>MGSSHHHHHHSSENLYFQGHSLPGANSLTIRKDSNKYVTAHFMVGIVENYTVDDWKHDMELAKETGIDAFALNCASIDSYTDKQLAYAYEAAEEVDFKVFISFDFAYWSNGDTARITSIMQTYADHPGQFQYNGAALVSTFVGDSFDWGPVKRAVDHPIFAVPNLQDPNWAGHATTSIDGAFSWYAWPTDGGNSIIKGPMTTIWDDRFRNNLKDKVYMAPVSPWFSTHFNTKNWVFICEDLPHLRWQQMLEMQPELIEIISWNDYGESHYIGPYSEAHSDDGSAQWTKDFPHDAWRIIAKPYIAAYKAGEREPTVESDQLVYWYRPTPKAVTCSKDPLGPPNGINLLEDSVFVTTLLTEPATLTVGSGSLEFSVDVDAGIVTNSFPMGVGSQAFSVTRDGEEILGGDGGLDVQDRCDYYNFNVYVGSFSA[5x]

Glycoside hydrolase family 71 (GH71) includes α-1,3-glucan degrading enzymes which could be exploited for biotechnological applications; however, the family is presently poorly understood. To increase our understanding of GH71, we have performed a phylogenetic analysis of the family and detailed biochemical analysis of two of the five GH71 enzymes encoded by Aspergillus nidulans (AnGH71B and -C). We present the first structure of a GH71 protein, AnGH71C, including structures with carbohydrate ligands. These structures revealed a conserved acidic dyad (DxxE), found to be crucial for activity, and active site water coordination consistent with a classical inverting GH mechanism.

Complexes of AnGH71C with glucose and nigerotriose/nigerotetraose were obtained by soaking crystals with ligand and clearly revealed the binding cleft within the N-terminal (β/α)8-barrel domain. The two protein molecules of the glucose-soaked crystals each contain two glucose molecules located in the same position in the binding cleft, while each of the four protein molecules of the nigerotetraose-soaked crystals contain distinct combinations of nigerotriose and nigerotetraose occupying different subsites within the cleft. Crystals of the apo protein and glucose-soaked crystals were of the C121 space group with similar unit cell dimensions and contained 2 molecules in the asymmetric unit, while the nigerotetraose soak was determined in P1 containing 4 molecules in the asymmetric unit. When overlaid and considered together, the annotation of the −4 to +3 subsites can be observed separated by two acidic residues (Asp265 and Glu268) found at the beginning of the loop between β8 and α8 of the (β/α)8-barrel domain. An additional nigerotriose molecule was also observed on the surface of the cleft in chain B extending from the +3 subsite and could be bound in +4, +5, and +6 subsites though the trisaccharide makes few direct interactions with the protein and its position on the surface of the cleft makes the subsite annotations questionable and could result from soaking ligand in high concentrations. Within different chains of the oligosaccharide-soaked crystal, both α- and β-anomers of nigerotetraose were observed occupying the -4 to -1 subsites. When the α-anomer is present, resembling the substrate configuration, a water molecule is positioned close to Asp265, 3.2 Å from the C1 atom of the sugar at the reducing end. This position is taken over by the hydroxyl of the β-anomer, the configuration of the inverted product. AnGH71C has an active site water molecule, proposed here to act as the catalytic nucleophile, positioned by the dyad’s aspartate in a small gap along the protein surface and in line with the C1 of α-anomer products. Only small protein structural changes are observed upon ligand binding in AnGH71C with the most significant being the packing of the loop between β6 and α6 over the substrate along the +1 to +3 sites leading to interactions with Gly193 and Asn194.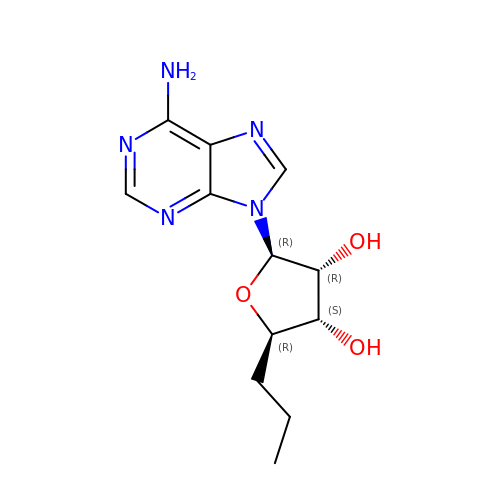(2~{R},3~{R},4~{S},5~{R})-2-(6-aminopurin-9-yl)-5-propyl-oxolane-3,4-diol | C12 H17 N5 O3 | BKDAOQOLDUJANJ-WOUKDFQISA-N> GMPFKQTRHLLTISALCPKELAYLIDRALDMKKNP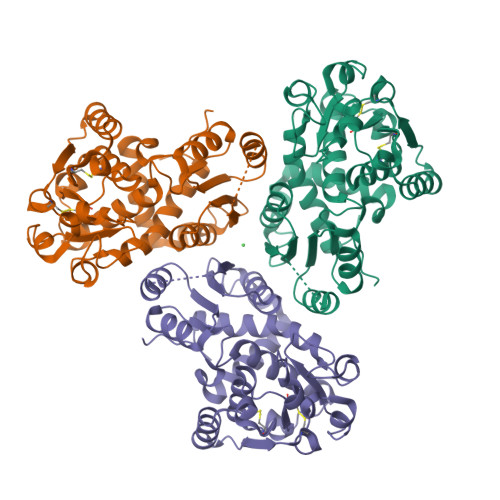AKYTARAANKTLLAFFAKPSLRTRVSLETAMTRLGGHAIYYELGANSNVGGKETVQDTAEVFSRMVDICTARLATKEMMREMAQHASVPCINALDDFGHPLQMVCDFMTIKEKFTAAGEFSNGFKGIKFAYCGDSMNNVTYDLMRGCALLGMECHVCCPDHKDFKPIKEVIDECEEIIAKHGTGGSIKIFHDCKKGCEGVDVVYTDSWMSYHITKEQKEARLKVLTPFQVDDAVMAVTSKRSIFMNCLPATRGEEQTASVIDGPKSVCYDEAGNRLHSAMAVLDFFLHDCKME>[3x]MFEARLVQGSILKKVLEALKDLINEACWDISSSGVNLQSMDSSHVSL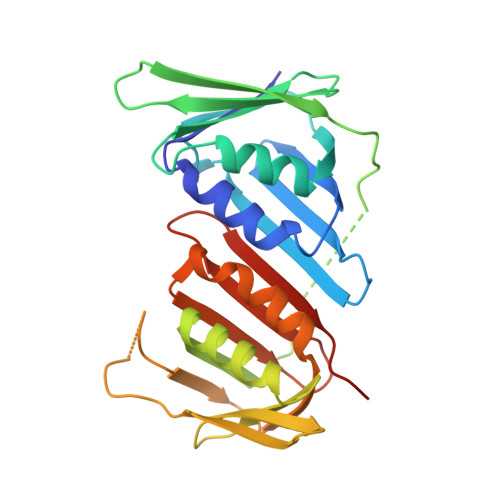VQLTLRSEGFDTYRCDRNLAMGVNLTSMSKILKCAGNEDIITLRAEDNADTLALVFEAPNQEKVSDYEMKLMDLDVEQLGIPEQEYSCVVKMPSGEFARISRDLSHIGDAVVISCAKDGVKFSASGELGNGNIKLSQTSNVDKEEEAVTIEMNEPVQLTFALRYLNFFTKATPLSSTVTLSMSADVPLVVEYKIADMGHLKYYLAPKIEDEEGS> GMSRTLVLFDIDGTLLKVESMNRRVLADALIEVYGTEGSTGSHDFSGKMDGAIIYEVLSNVGLERAEIADKFDKAKETYIALFRERARREDITLLEGVRELLDALSSRSDVLLGLLTGNFEASGRHKLKLPGIDHY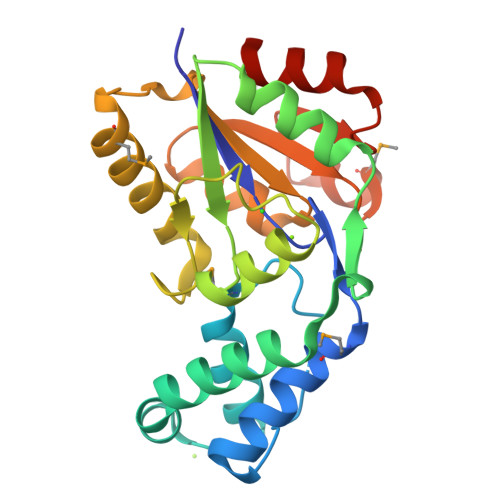FPFGAFADDALDRNELPHIALERARRMTGANYSPSQIVIIGDTEHDIRCARELDARSIAVATGNFTMEELARHKPGTLFKNFAETDEVLASILTPKHS>[2x]ASQNSFRIEYDTFGELKVPNDKYYGAQTVRSTMNFKIGGVTERMPTPVIKAFGILKRAAAEVNQDYGLDPKIANAIMKAADEVAEGKLNDHFPLVVWQTGSGTQTNMNVNEVISNRAIEMLGGELGSKIPVHPNDHVNKSRSSNDTFPTAMHIAAAIEVHEVLLPGLQKLHDALDAKSKEFAQIIKIGRTHTQDAVPLTLGQEFSGYVQQVKYAMTRIKAAMPRIYELAAGGTAVGTGLN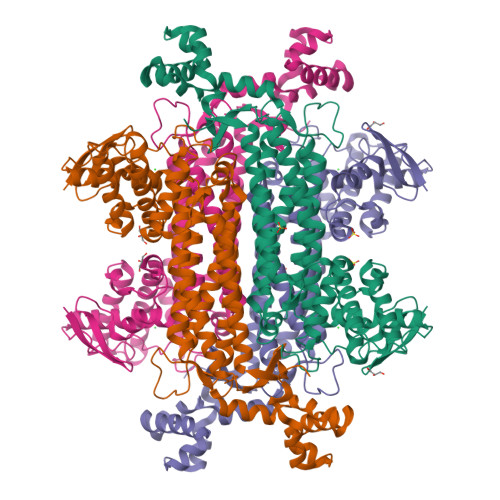TRIGFAEKVAAKVAALTGLPFVTAPNKFEALAAHDALVELSGAMNTTACSLMKIANDIRFLGSGPRSGLGELILPENEPGSSIMPGKVNPTQCEAMTMVAAQVMGNHVAVTVGGSNGHFELNVFKPMMIKNVLHSARLLGDASVSFTENCVVGIQANTERINKLMNESLMLVTALNPHIGYDKAAKIAKTAHKNGSTLKETAIELGYLTAEQFDEWVKPKDMLGPK> LERN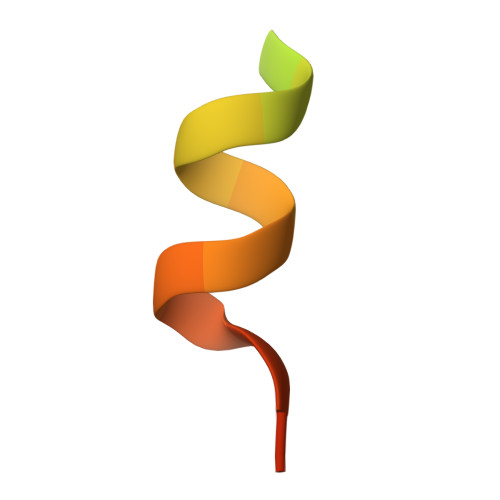NIKQAANNSLLLHLLKSQTIP>[3x]PPGPP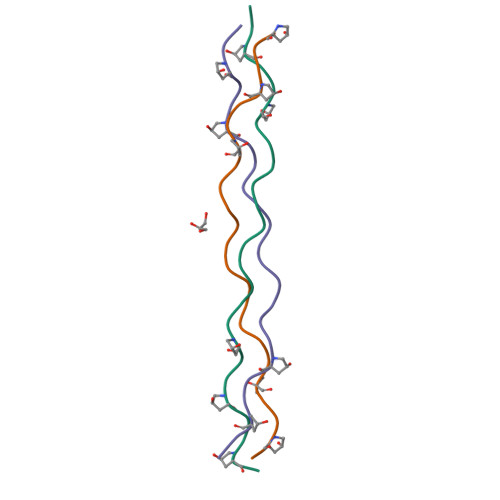GPPGEKGERGYPGPPGPPGPPG> RRMDRENEGSLRVLMLPWLAHGHISPFLELAKRLAKKNFHIYLCSTPINLSSIKK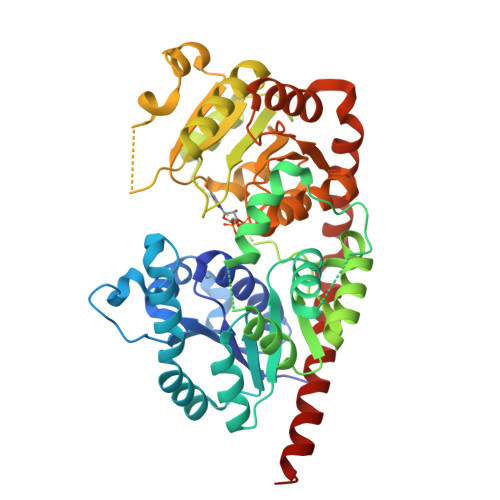TISQEYSLSIQLVELPLPSLPDLPPQYHTTNGLPPHLMPTLKRAYEMSSPTFSNILKTLLPDLLIYDFNQMWAVDTATSLNIPSVQFSTTGTITASFAMYMLKNPDSENAKYPFPEIYLWEYELERMRKAWVESSKVSDSNEGDQLLECASKSCGIILIKSFRELEGKYIDFFSELSGKKIVPVGPLVQESLDDQDEKGEIIQWLDKKDKSSVVFVSFGSEYFLTSEEMEEIAHGLESGNVNFIWVLRFPVGKKISVAEALPKGFLERIGDRGMVVEGWAPQAKILKHSSTGGFVSHCGWSSIMESMKLGIPIIAMPMQLDQPFNARLLEEFGVAMEVVREKDGTLRREEIANVIRKVVVEKSGEGVRAKARQVSESLRKKGDEEVDEVVVELLQICRKYELIGKMSTLR> MSMTILPLELIDKCIGSNLWVIMKSEREF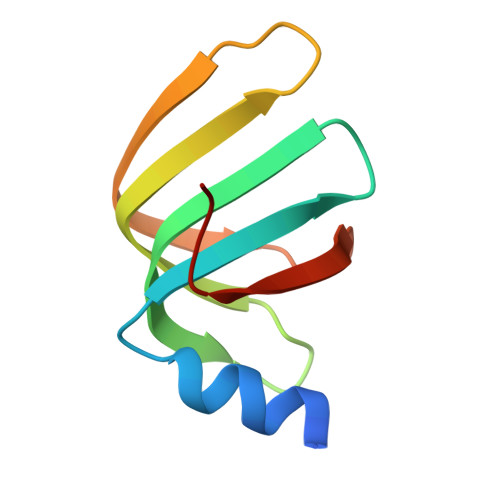AGTLVGFDDYVNIVLKDVTEYDTVTGVTEKHSEMLLNGNGMCMLIPGGKPE>[2x]MFNSDNLRLDGKCAIITGAGAGIGKEIAITFATAGASVVVSDINADAANHVVDEIQQLGGQAFACRCDITSEQELSALADFAISKLGKVDILVNNAGGGGPKPFDMPMADFRRAYELNVFSFFHLSQLVAPEMEKNGGGVILTITSMAAENKNINMTSYASSKAAASHLVRNMAFDLGEKNIRVNGIAPGAILTDALKSVITPEIEQKML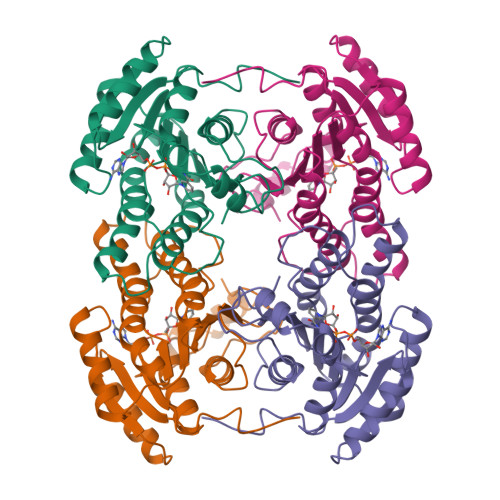QHTPIRRLGQPQDIANAALFLCSPAASWVSGQILTVSGGGVQELN> GLPTTTLPGSGQFLTTDDRQSPSALPNYEPTPRIHIPGKV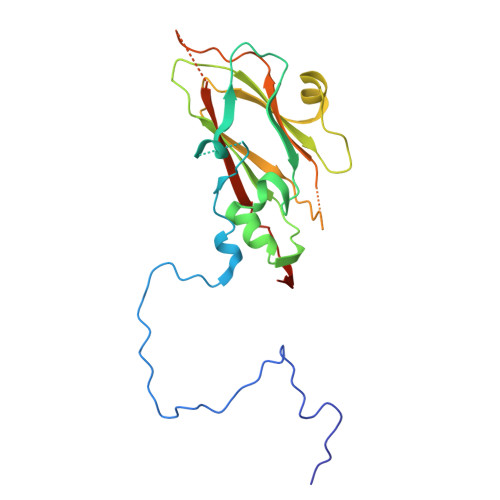HNLLEIIQVDTLIPMNNTHTKDEVNSYLIPLNANRQNEQVFGTNLFIGDGVFKTTLLGEIVQYYTHWSGSLRFSLMYTGPALSSAKLILAYTPPGARGPQDRREAMLGTHVVWDIGLQSTIVMTIPWTSGVQFRYTDPDTYTSAGFLSCWYQTSLILPPETTGQVYLLSFISACPDFKLRLMKDTQTISQTV>[3x]PARSVVALKTPIKVELVAGKTYRWCVCGRS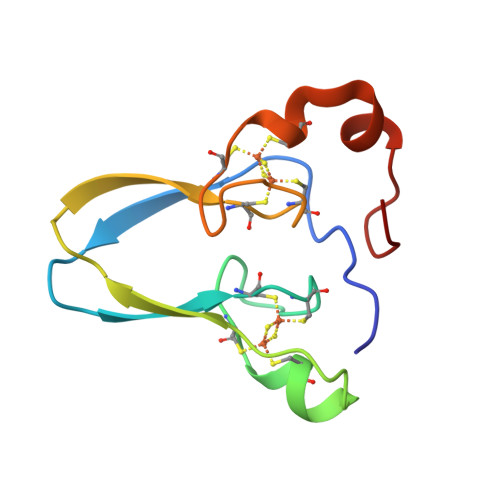KKQPFCDGSCFFQRTGLSPLKFKAQETRMVALCTCKATQRPPYCDGTCRSERVQKAEVGSPL> SMAATAAEAVASGSGEPREEAGALGPAWDESQLRSYSFPTRPIPRLSQSDPRAEELIENEEPVVLTDTNLVYPALKWDLEYLQENIGNGDFSVYSASTHKFLYYDEKKMANFQNFKPRSNREEMKFHEFVEKLQDIQQRGGEERLYLQQTLNDTVGRKIVMDFLGFNWNWINKQQGKRGWGQLTSNLLLIGMEGNVTPAHYDEQQNFFAQI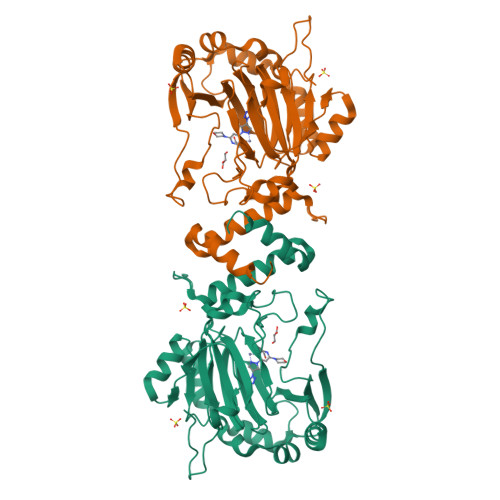KGYKRCILFPPDQFECLYPYPVHHPCDRQSQVDFDNPDYERFPNFQNVVGYETVVGPGDVLYIPMYWWHHIESLLNGGITITVNFWYKGAPTPKRIEYPLKAHQKVAIMRNIEKMLGEALGNPQEVGPLLNTMIKGRYN> YKVERNPPAFTELQLPRYIMAGFPVCPKLSLEFGDPASSLFRWYKEAKPGAAEPEVGVPSSLSPSSPSSSWTETDVEERVYTPSNADIGLRLKLHCTPGDGQRFGHSRELESVCVVEAGPGTCTFDHRHLYTKKVTEDALIRTVSYNILADTYAQTEFSRTVLYPYCAPYALELDYRQNLIQKELTGYNADVICLQEVDRAVFSDSLVPALEAFGLEGVFRIKQHEGLATFYRKSKFSLLSQHDISFYEALESDPLHKELLEKLVLYPSAQEKVLQRSSVLQVSVLQSTKDSSKRICVANTHLYWHPKGGYIRLIQMAVALAHIRHVSCDLYPGIPVIFCGDFNSTPSTGMYHFVINGSIPEDH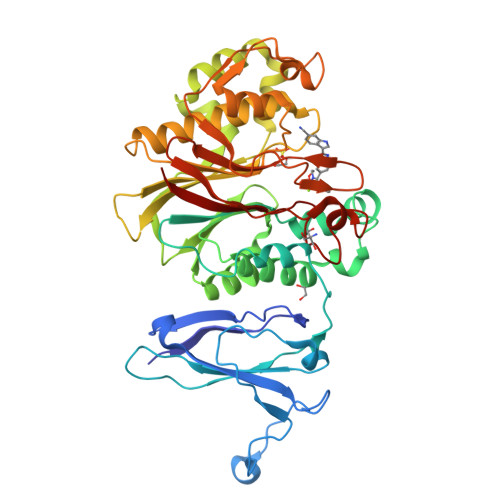EDWASNGEEERCNMSLTHFFKLKSACGEPAYTNYVGGFHGCLDYIFIDLNALEVEQVIPLPSHEEVTTHQALPSVSHPSDHIALVCDLKWK> MSMLVVVTENVPPRLRGRLAIWLLEVRAGVYVGDVS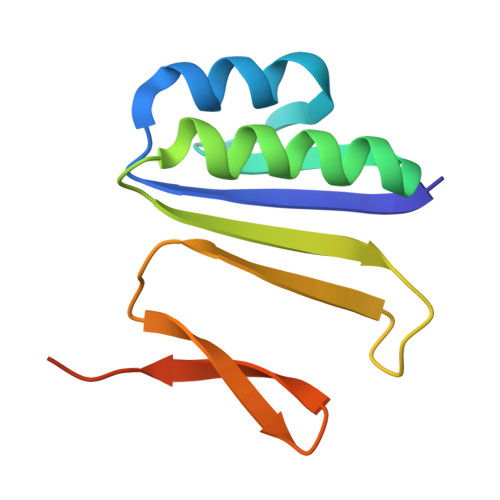AKIREMIWEQIAGLAEEGNVVMAWATNTETGFEFQTFGLNRRTPVDLDGLRLVSFLPVGSSENLYFQ>MSDMKHSKLLILGSGPAGYTAAVYAARANLNPVLITGMQQGGQLTTTTEVENWPGDPEGLTGPGLMDRMKEHAERFETEIIFDHINEVDFSTRPFVLKGDAASYSCDALIISTGASAKYLGLESEEAFKGRGVSACATCDGFFYRNQKVAVVGGGNTAVEEALYLSNIAAEVHLIHRRDSFRAEKILINRLMDKVQNGNIVLHTDRVLDEVLGDEMGVTGVRLKDVKTGGTEELDVMGAFIAIGHSPNTQIFQGQ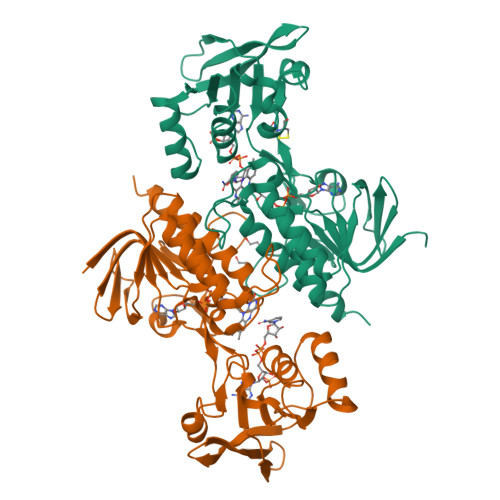LDMKDGYILVKSGLEGNATQTSVEGIFAAGDVMDHNYRQAITSAGTGCMAALDAERYLDSLNDK[2x]>MSFMDQIPGGGNYPKLPVECLPNFPIQPSLTFRGRNDSHKLKNFISEIMLNMSMISWPNDASRIVYCRRHLLNPAAQWANDFVQEQGILEITFDTFIQGLYQHFYKPPDINKIFNAITQLSEAKLGIERLNQRFRKIWDRMPPDFMTEKAAIMTYTRLLTKETYNIVRMHKPETLKDAMEEAYQTTALTERFFPGFELDADGDTIIGATTHLQEEYDSDYDSEDNLTQNRYVHTVRTRRSYNKPMSNHRNRRNNNASREECIK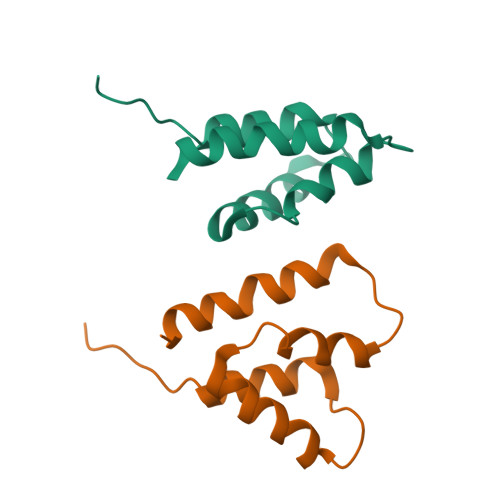NRLCFYCKKEGHRLNECRARKAVLTDLELESKDQQTLFIKTLPIVH[2x]>[2x]GMADEATRRVVSEIPVLKTNAGPRDRELWVQRLKEEYQSLIRYVENNKNADNDWFRLESNKEGTRWFGKCWYIHDLLKYEFDIEFDIPITYPTTAPEIAVPELDGKTAKMYRGGKICLTDHFKPLWARNVPKFGLAHLMALGLGPWLAVEIPDLIQKGVIQHKEKCNQ;>DSGESLEDLMAKMKNM[2x]

Analogous to ubiquitination, ufmylation is carried out by a three-enzyme cascade involving E1, E2, and E3 proteins. The E1 UBA5 has three distinct regions: (1) an adenylation domain that binds ATP and magnesium ions; (2) a UFM1-interacting sequence (UIS) spanning amino acids 334 to 346 that holds UFM1 in a trans binding mechanism; and (3) a UFC1-binding sequence (UBS) from 392 to 404 that binds UFC117–21. The adenylated UFM1 is then subjected to a nucleophilic attack by the catalytic C250 of UBA5 to form a thioester bond with the C-terminal glycine of UFM1. This is followed by a trans thiolation process, whereby the UFM1 is transferred to the E2 UFC1 forming a thioester bond with C116 of UFC1. However, UBA5 does not harbor such a domain but instead has a short sequence called UBS that is responsible for the interaction with UFC128.

Here we report the crystal structure of UFC1 in complex with the UBS of UBA5. This structure reveals that the UBS adopts a helical conformation that interacts with UFC1, mainly via hydrophobic interactions. The UBS forms an α-helix and interacts with UFC1 on the side opposite to the active site surface. The UBS residues L394, L397, M398, M401, and M404 form hydrophobic interactions with residues V29, L32, L39, I40, V43 of α-helix 1 and F54 and L56 of β-strand 1 of UFC1. More specifically, M401 occupies a hydrophobic pocket on the UFC1 surface. Accordingly, M401R and L397R mutations in the UBS prevented the interaction with UFC1 and damaged UFM1 transfer. Besides hydrophobic interactions, the main chain carboxyl oxygen atoms of M404 forms hydrogen bonds with the side chains of UFC1 K47 and R55. In addition, K400 and K402 of the UBS form salt bridges with E44 and E57 of UFC1, respectively. However, mutations of these residues did not affect UFM1 transfer, suggesting that the binding of UBS to UFC1 is mainly mediated by hydrophobic interactions. UFC1 possesses a pocket, lacking in other E2 enzymes, in which the UBS fits spatially.>[2x]MGHHHHHHHHHHSSGHIEGRHMMAERKGTAKVDFLKKIEKEIQQKWDTERVFEVNASNLEKQTSKGKYFVTFPYPYMNGRLHLGHTFSLSKCEFAVGYQRLKGKCCLFPFGLHCTGMPIKACADKLKREIELYGCPPDFPDEEEEEEETSVKTEDIIIKDKAKGKKSKAAAKAGSSKYQWGIMKSLGLSDEEIVKFSEAEHWLDYFPPLAIQDLKRMGLKVDWRRSFITTDVNPYYDSFVRWQFLTLRERNKIKFGKRYTIYSPKDGQPCMDHDRQTGEGVGPQEYTLLKLKVLEPYPSKLSGLKGKNIFLVAATLRPETMFGQTNCWVRPDMKYIGFETVNGDIFICTQKAARNMSYQGFTKDNGVVPVVKELMGEEILGASLSAPLTSYKVIYVLPMLTIKEDKGTGVVTSVPSDSPDDIAALRDLKKKQALRAKYGIRDDMVLPFEPVPVIEIPGFGNLSAVTICDELKIQSQNDREKLAEAKEKIYLKGFYEGIMLVDGFKGQKVQDVKKTIQKKMIDAGDALIYMEPEKQVMSRSSDECVVALCDQWYLDYGEENWKKQTSQCLKNLETFCEETRRNFEATLGW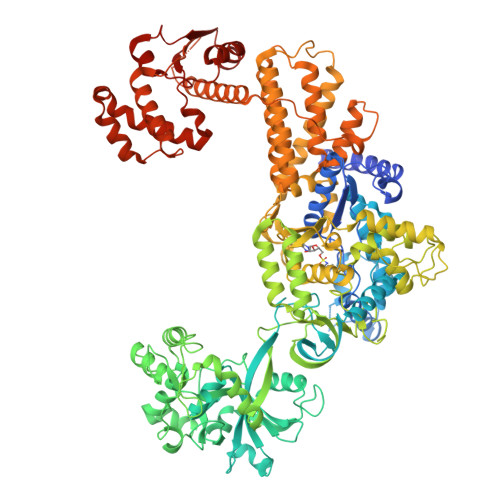LQEHACSRTYGLGTHLPWDEQWLIESLSDSTIYMAFYTVAHLLQGGNLHGQAESPLGIRPQQMTKEVWDYVFFKEAPFPKTQIAKEKLDQLKQEFEFWYPVDLRVSGKDLVPNHLSYYLYNHVAMWPEQSDKWPTAVRANGHLLLNSEKMSKSTGNFLTLTQAIDKFSADGMRLALADAGDTVEDANFVEAMADAGILRLYTWVEWVKEMVANWDSLRSGPASTFNDRVFASELNAGIIKTDQNYEKMMFKEALKTGFFEFQAAKDKYRELAVEGMHRELVFRFIEVQTLLLAPFCPHLCEHIWTLLGKPDSIMNASWPVAGPVNEVLIHSSQYLMEVTHDLRLRLKNYMMPAKGKKTDKQPLQKPSHCTIYVAKNYPPWQHTTLSVLRKHFEANNGKLPDNKVIASELGSMPELKKYMKKVMPFVAMIKENLEKMGPRILDLQLEFDEKAVLMENIVYLTNSLELEHIEVKFASEAEDKIREDCCPGKPLNVFRIEPGVSVS> ASEEEKAWLMASRQQLAKETSNFGFSLLRKISMRHDGNMVFSPFGMSLAMTGLMLGATGPTETQIKRGLHLQALKPTKPGLLPSLFKGLRETLSRNLELGLTQGSFAFIHKDFDVKETFFNLSKRYFDTECVPMNFRNASQAKRLMNHYINKETRGKIPKLFDEINPETKLILVDYILFKGKWLTPFDPVFTEVDTFHLDKYKTIKVPMMYGAGKFASTFDKNFRCHVLKLPYQGNATMLVVLMEKMGDH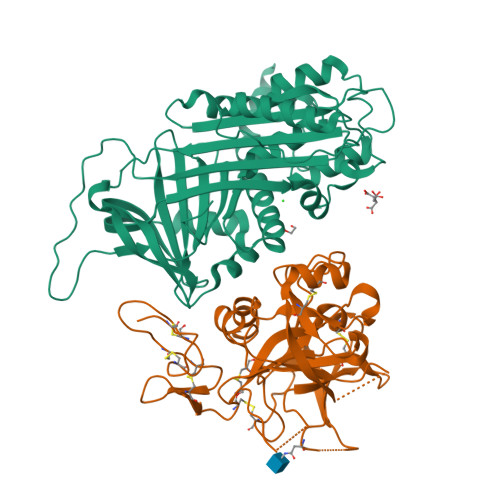LALEDYLTTDLVETWLRNMKTRNMEVFFPKFKLDQKYEMHELLRQMGIRRIFSPFADLSELSATGRNLQVSRVLQRTVIEVDERGTEAVAGILSEITAYSMPPVIKVDRPFHFMIYEETSGMLLFLGRVVNPTLL;> AKNECHPERTDGCQHFCLPGQESYTCSCAQGYRLGEDHKQCVPHDQCACGVLTSEKRAPDLQDLPWQVKLTNSEGKDFCGGVIIRENFVLTTAKCSLLHRNITVKTYFNRTSQDPLMIKITHVHVHMRYDADAGENDLSLLELEWPIQCPGAGLPVCTPEKDFAEHLLIPRTRGLLSGWARNGTDLGNSLTTRPVTLVEGEECGQVLNVTVTTRTYCERSSVAAMHWMDGSVVTREHRGSWFLTGVLGSQPVGGQAHMVLVTKVSRYSLWFKQIMNAHHHHHH>[2x]MQTEHVILLNAQGVPTGTLEKYAAHT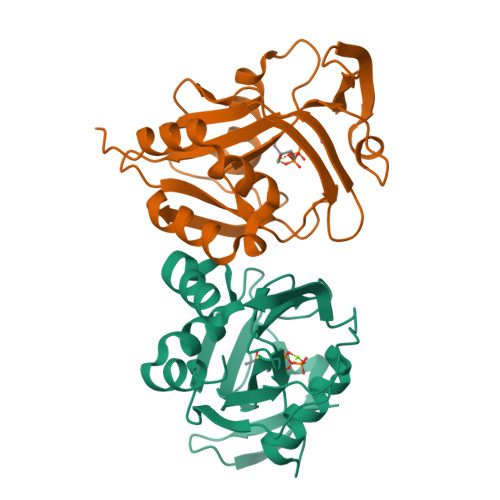ADTRLHLAFSSWLFNAKGQLLVTRRALSKKAWPGVWTNSVCGHPQLGESNEDAVIRRCRYELGVEITPPESIYPDFRFRATDPSGIVENEVCPVFAARTTSALQINDDEVMDYQWCDLADVLHGIDATPWAFSPWMVMQATNREARKRLSAFTQLKLHHHHHH>[2x]ASSVNELENWSKWMQPIPDNIPLARISIPGTHDSGTFKLQNPIKQVWGMTQEYDFRYQMDHGARIFDIRGRLTDDNTIVLHHGPLYLYVTLHEFINEAKQFLKDNPSETIIMSLKKEYEDMKGAEGSFSSTFEKNYFVDPIFLKTEGNIKLGDARGKIVLLKRYSGSNESGGYNNFYWPDNETFTTTVNQNVNVTVQDKYKVNYDEKVKSIKDTMDE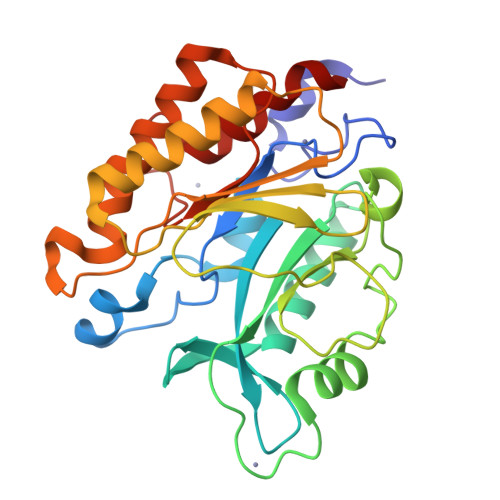TMNNSEDLNHLYINFTSLSSGGTAWNSPYSYASSINPEIANDIKQKNPTRVGWVIQDYINEKWSPLLYQEVIRANKSLIKE>AQNYFGSINISNANVKQAVWFAMKEYNKESEDKYVFLVDKILHAKLQITDRMEYQIDVQISRSNCKK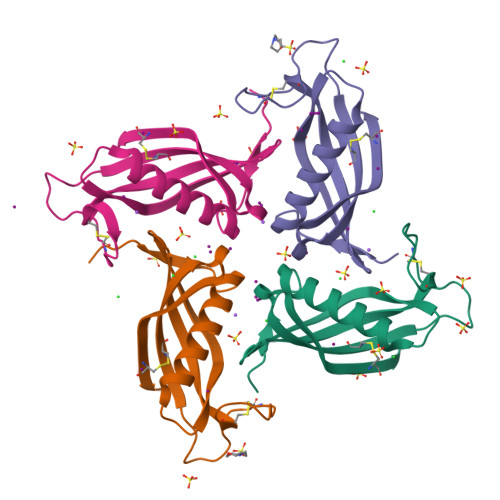PLNNTENCIPQKKPELEKKMSCSFLVGALPWNGEFNLLSKECKDV[4x]GAMMA-D-GLUTAMIC ACID | C5 H9 N O4 | 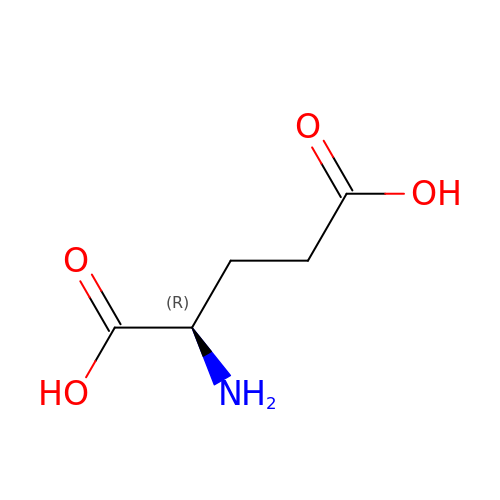WHUUTDBJXJRKMK-GSVOUGTGSA-N>[4x]NVIIGNQKLTINDVARVARNGTLVSLTNNTDILQGIQASCDYINNAVESGEPIYGVTSGFGGMANVAISREQASE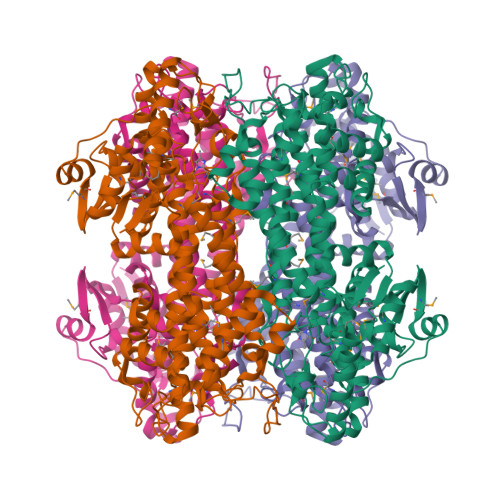LQTNLVWFLKTGAGNKLPLADVRAAMLLRANSHMRGASGIRLELIKRMEIFLNAGVTPYVYEFGSIGASGDLVPLSYITGSLIGLDPSFKVDFNGKEMDAPTALRQLNLSPLTLLPKEGLAMMNGTSVMTGIAANCVYDTQILTAIAMGVHALDIQALNGTNQSFHPFIHNSKPHPGQLWAADQMISLLANSQLVRDELDGKHDYRDHELIQDRYSLRCLPQYLGPIVDGISQIAKQIEIEINSVTDNPLIDVDNQASYHGGNFLGQYVGMGMDHLRYYIGLLAKHLDVQIALLASPEFSNGLPPSLLGNRERKVNMGLKGLQICGNSIMPLLTFYGNSIADRFPTHAEQFNQNINSQGYTSATLARRSVDIFQNYVAIALMFGVQAVDLRTYKKTGHYDARASLSPATERLYSAVRHVVGQKPTSDRPYIWNDNEQGLDEHIARISADIAAGGVIVQAVQDILPS As a proof of concept, we used this platform to identify both known and novel L- and D-amino acid peptide binders to the well-characterized model target, streptavidin. All peptides bind within or near the biotin binding pocket of streptavidin formed by two surface loops [1/2 (amino acids 22–28) and 3/4 (amino acids 42–52)], and by antiparallel β-sheets involved in an extensive polar interaction network, in which residues Ser88 and Thr90 of β-strand 6 play a major role. The surface loops of streptavidin are flexible: upon biotin binding they undergo a conformational change to form a closed conformation, but to accommodate the peptide ligands, loop 3/4 is dislocated by 13–16 Å from the biotin closed form to adopt a well-defined peptide-specific structure. All eight L- and D-peptides discovered in this work bind to the same pocket of streptavidin in distinctive binding modes suggesting (1) the rich malleability of L- and D-peptides and (2) the ability of streptavidin itself to adjust the flexible loop to accommodate multiple peptides with diverse sequences and conformations.

Most selected sequences (1,019 of 1,100) contained HP, PQ, or PM sequences: their presence would be expected in the well-known HPQ and HPM streptavidin binders. Binding conformation of EWVHPQFEQKAK peptide closely resembles previously published HPQ peptide-streptavidin structures. The HPQFE amino acids at positions 4–8, occupy the biotin-binding pocket of streptavidin and adopt a rigid conformation, whereas the N- and C-terminal amino acids are exposed to the solvent and show significant degree of freedom in the crystal structure [Fig. 4(B)]. The His4 and Gln6 sidechains of the HPQ motif form hydrogen bonds with residues Ser88 and Thr90 of streptavidin. Pro5 is crucial for positioning the Gln6 sidechain within hydrogen bonding distance of Thr90. The sidechain of Phe7 is involved in critical π-π stacking against Trp120 from a neighboring streptavidin subunit. To explain why “secondary” binders that exhibit higher affinity to streptavidin than the commonly reported HPQ-motif binders have not been previously selected in random libraries, we assumed that the HPQ(M) motif contributes most of the binding energy, whereas the contribution of the flanking sequences is relatively minor and multiple flanking sequences are acceptable.

>[8x]MRKIVVAAIAVSLTTVSITASASADPSKDSKAQVSAAEAGITGTWYNQLGSTFIVTAGADGALTGTYESAVGNAESRYVLTGRYDSAPATDGSGTALGWTVAWKNNYRNAHSATTWSGQYVGGAEARINTQWLLTSGTTEANAWKSTLVGHDTFTKVKPSAASIDAAKKAGVNNGNPLDAVQQ;>[8x]EWVHPQFEQKAK>[2x]AMDPEFMREFQRAAVRLHILHHAADNEVHGAW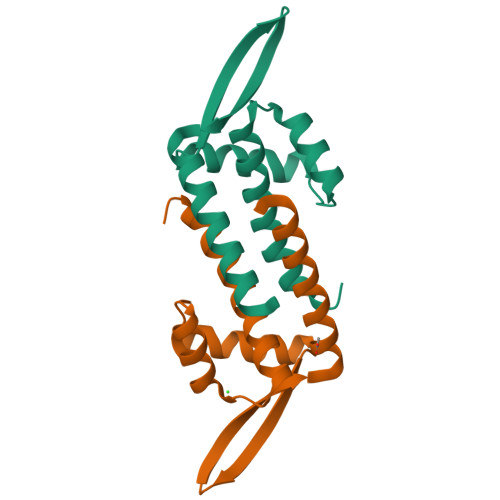LTQELSRHGYRVSPGTLYPTLHRLEADGLLVSEQRVVDGRARRVYRATPAGRAALTEDRRALEELAREVLGGQSHTAGNGT>SASTSGNPFQANVEMKTFMERFNLTHHHQSGIYVDLGQDKEVDGTLYREPAGLCPIWGKHIELQQPDRPPYRNNFLEDVPTEKEYKQSGNPLPGGFNLNFVTPSGQRISPFPMELLEKNSNIKASTDLGRCAEFAFKTVAMDKNNKATKYRYPFVYDSKKRLCHILYVSMQLMEGKKYCSVKGEPPDLTWYCFKPRKSVTENHHLIYGSAYVGENPDAFISKCPNQALRGYRFGVWKKGRCLDYTELTDTVIERVESKAQCWVKTFENDGVASDQPHTYPLTSQASWNDWWPLHQSDQPHSGGVGR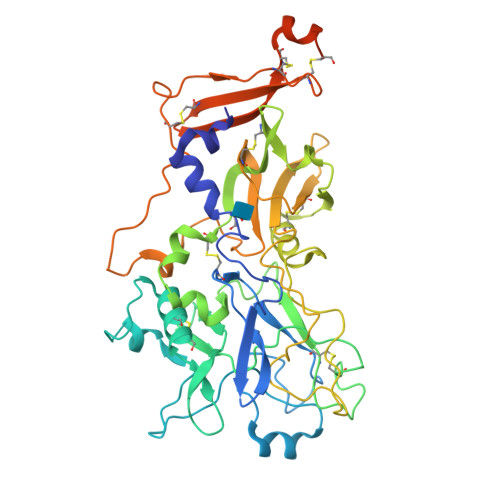NYGFYYVDTTGEGKCALSDQVPDCLVSDSAAVSYTAAGSLSEETPNFIIPSNPSVTPPTPETALQCTADKFPDSFGACDVQACKRQKTSCVGGQIQSTSVDCTADEQNECGSNTALIAGLAVGGVLLLALLGGGCYFAKRLDRNKGVQAA[4x]> MGSSHHHHHHHHSSGLEVLFQGPLGSHMNTRRQQAQNIRNNAAELAANRPHPQHINNKEEYEYRRPKKDGNEPSHIANFTKGLPHDEHTGLLLNSADYDQFVLGIQSGDTTDFARTPLGPAELPKVHGCLSKQKIDCDDDHRSGFWKSQIAQGAAGGDGAKLRAWESAGAGLVFDLEGPDAQAVTMPPAPRLESPELTSEIAEVYSQALLRDIHFSQLRDPGLGDQVNACDSCPTQLSIYEAIDILNTVQIEGQNWFSANCCDLTDDEQARQRPLVTRQNIFRGIAPGDDVGPYLSQFLLIGNNALGGGVFGQEAGHIGYGAIRIDQRVRKATPCKDFMTNFETWLDVQNGADLRGLETYVDADPGKCREFPAYRVITTPRDLATYVHYDALYEAYLNACLILLGMGAPFDPGIPFQKPDVEDKQQGFAHFGGPQILTLVCEAATRGLKAVSFQKFNVHRRLRPEALGGLVDRYKHGKGAGDELKPVAALVEALENVGLLSKVVAHNQLQNQNLDRSGDPSSAGDNYFLPMAFPEGSPMHPSYGAGHATVAGACVTMLKAFFDHGWQLNLGMANGKYISYEPNQDGSSLQQVLLDCPLTVEGELNKIAANISIGRDWAGVHYFTDYIESLRLGEKIAIGILEEQKLTYGENFTMTVPLYDGGSIQI

Vanadium-dependent haloperoxidases (VHPOs) are biotechnologically valuable and operationally versatile biocatalysts. VHPOs are categorized according to the most electronegative halide they can oxidize, leading to chloroperoxidases (VCPOs), bromoperoxidases (VBPOs), and iodoperoxidases (VIPOs). The general mechanism for VHPO-catalyzed reactions is based on the two-electron oxidation of halides. For elucidating the halogen specificity in VHPOs, we chose the vanadium-dependent haloperoxidase AmVHPO from the cyanobacterium Acaryochloris marina MBIC 1101721.

Mutagenesis experiments in the second shell combined with activity screening assays revealed that R425S-VCPO was transformed into a chloroperoxidase capable of efficient aromatic chlorination, even on a preparative scale. Strikingly, the conversion of 3 by bromination and chlorination drastically increased from 53% for bromination and 8% for chlorination for the wild-type AmVHPO to 91% and 74%, respectively, for the R425S variant. An isosteric phosphate, obtained from the reservoir solution, replaced the cofactor vanadate in the enzyme crystals. Both mutant structures feature the identical characteristic assembly of a hexamer of dimers, arranged in a “head-to-tail” orientation with superimposable key catalytic residues when compared to the wild-type. In detail, residues 390–404 in the wild-type structure lack a defined electron density due to flexibility. In contrast, in R425S, this section consolidated in a loop structure, strongly influenced by the introduced serine residue (highlighted in blue). Remarkably, variant R425S showed an interaction between Ser425 and a region of the adjacent subunit (highlighted in blue). Exchanging Arg425 by serine organizes residues 390–404 in R425S to a defined loop. This structural variation has no immediate influence on its protein subunit but causes mutual interactions of two neighboring monomers in the ‘head-to-tail´ orientation of the dodecameric enzyme structure. Consequently, the loop triggers the formation of a defined tunnel with the vanadate cofactor at the end. Although the key catalytic residues in the first coordination sphere of cofactor binding are still strictly conserved within the R425S-AmVHPO mutant, the Ser425 from the adjacent subunit alters the hydrogen-bonding network within the active site, thus forming a tunnel protecting the vanadate in the active site.> MSPFPLTSMDKAFITVLEMTPVLGTEIINYRDGMGRVLAQDVYAKDNLPPFPASVKDGYAVRAADGPGDRFIIGESQAGEQPTQTVMPGQVMRVTTGAPIPCGADAVVQVEDTELIRESDDGTEELEVRILVQARPGQDIRPIGHDIKRGECVLAKGTHMGPSEIGLLATVGVTEVEVNKFPVVAVMSTGNELLNPEDDLLPGKIRDSNRSTLLATIQEHGYPTINLGIVGDNPDDLLNALNEGISRADVIITSGGVSMGEKDYLKQVLDIDLHAQIHFGRVFMKPGLPTTFATLDIDGVRKII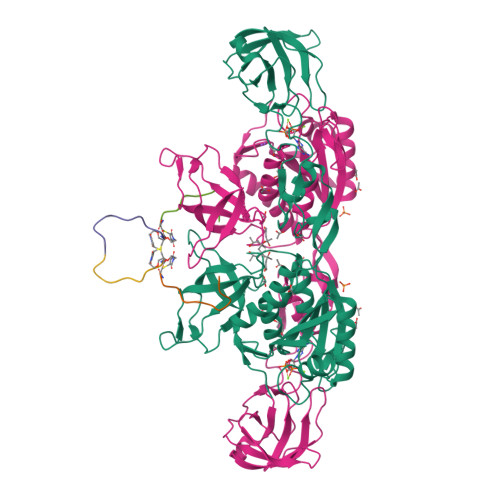FALPGNPVSAVVTCNLFVVPALRKMQGILDPRPTIIKARLSCDVKLDPRPEYHRCILTWHHQEPLPWAQSTGNQMSSRLMSMRSANGLLMLPPKTEQYVELHKGEVVDVMVIGRL;>FNIVGTTYPC[2x]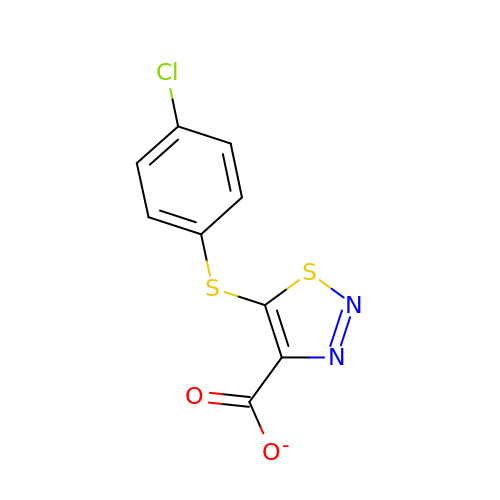5-[(4-chlorophenyl)sulfanyl]-1,2,3-thiadiazole-4-carboxylate | C9 H4 Cl N2 O2 S2 | NDYKFFAREALEPX-UHFFFAOYSA-M> MILLDTNVISEPLRPQPNERVVAWLDSLILEDVYLSAITVAELRLGVALLLNGKKKNVLHERLEQSILPLFAGRIL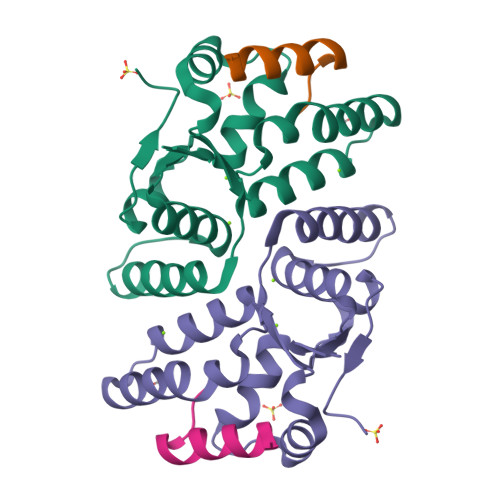PFDEPVAAIYAQIRSYAKTHGKEIAAADGYIAATAKQHSLTVATRDTGSFFAADVAVFNPWHL;> VRLGSMLASIGQEIGGVEL>[2x]GHHHHHHHHGSS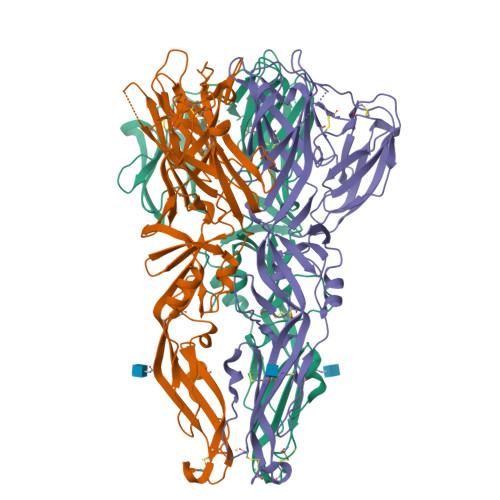TSNGMRCVGIGNRDFVEGLSGATWVDVVLEHGSCVTTMAKDKPTLDIELLKTEVTNPAVLRKLCIEAKISNTTTDSRCPTQGEATLVEEQDTNFVCRRTFVDRGHGNGCGLFGKGSLITCAKFKCVTKLEGKIVQYENLKYSVIVTVHTGDQHQVGNETTEHGTIATITPQAPTSEIQLTDYGALTLDCSPRTGLDFNEMVLLTMEKKSWLVHKQWFLDLPLPWTSGASTSQETWNRQDLLVTFKTAHAKKQEVVVLGSQEGAMHTALTGATEIQTSGTTTIFAGHLKCRLKMDKLTLKGMSYVMCTGSFKLEKEVAETQHGTVLVQVKYEGTDAPCKIPFSSQDEKGVTQNGRLITANPIVTDKEKPVNIEAEPPFGESYIVVGAGEKALKLSWFKKGSSIGKMFEATARGARR>MLEKKRVSFRPMNEDDLVLMLKWLTDDRVLEFYDGRDKKHTQKTIREHYTEQWADEIYRVIIEYDTIPIGYAQIYRIQGELFDEYNYHETEEKIYAMDQFIGEPEYWNMGIGAEYCRVVCQYLRTEMDADAVILDPRKNNLRAVRAYQKAGFKIIKELPEHELHEG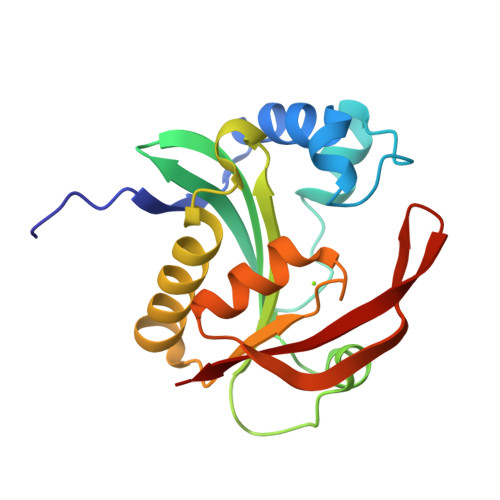KKEDCVLMEWRV[2x]>TITLTENKRKSMEKLSVDGVISALAFDQRGALKRMMAQHQTKEPTVEQIEELKSLVSEELTPFASSILLDPEYGLPASRVRSEEAGLLLAYEKTGYDATTTSRLPDCLDVWSAKRIKEAGAEAVKFLLYYDIDGDQDVNEQKKAYIERIGSECRAEDIPFYLEILTYDEKIADNASPEFAKVKAHKVNEAMKVFSKERFGVDVLKVEVPVNMKFVEGFADGEVLFTKEEAAQAFRDQEASTDLPYIYLSAGVSAKLFQDTLVFAAESGAKFNGVLCGRATWAGSVKVYIEEGPQAAREWLRTEGFKNI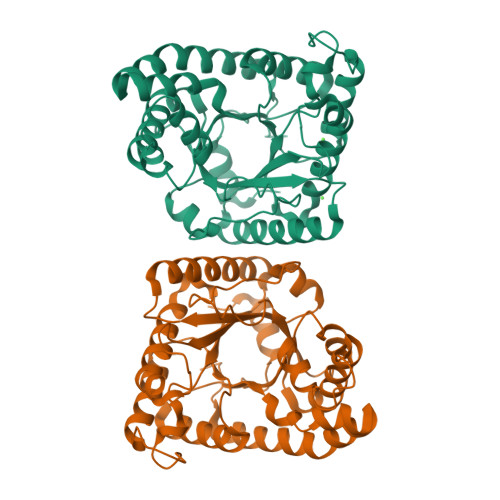DELNKVLDKTASPWTEKM[4x]>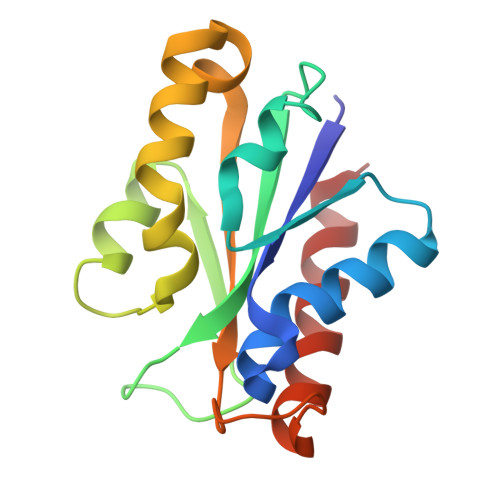[2x]MRVLILALGNELMKDDGAGLKAGRILAEKGYNVLEVGTDIFRLANHYNGEERIVIIDAILSDKLKPGEVVHFSGEEIFEKLKAEIRSAHFMGAIDGLKLLMALDERLKRAEIHFIGIVAKEIDLGMELSDEVKAGVQKAVEIAEKLAK> ANIVGGIEYSINNASLCSVGFSVTRGATKGFVTAGHCGTVNATARI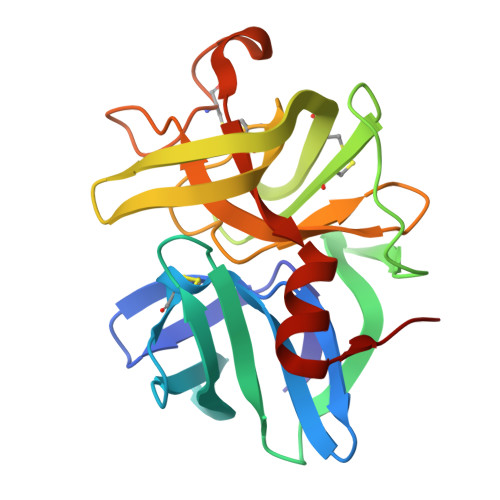GGAVVGTFAARVFPGNDRAWVSLTSAQTLLPRVANGSSFVTVRGSTEAAVGAAVCRSGRTTGYQCGTITAKNVTANYAEGAVRGLTQGNACMGRGDSGGSWITSAGQAQGVMSGGNVQSNGNNCGIPASQRSSLFERLQPILSQYGLSLVTG(4~{S})-4-[(2~{R})-3-[(4-azanyl-2-methyl-pyrimidin-5-yl)methyl]-4-methyl-5-[2-[oxidanyl(phosphonooxy)phosphoryl]oxyethyl]-2~{H}-1,3-thiazol-2-yl]-4-oxidanyl-4-phosphono-butanoic acid | C16 H27 N4 O13 P3 S | 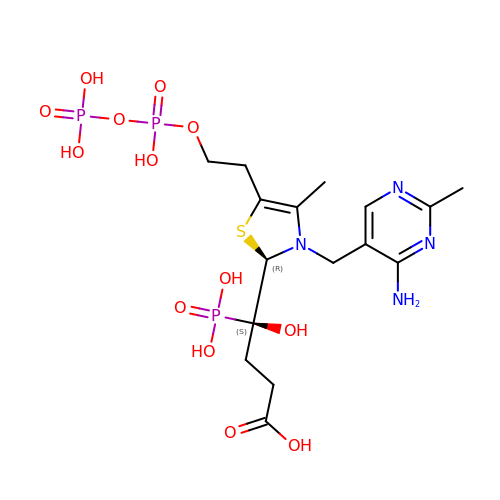XWZWGSGHSWWOAH-CVEARBPZSA-N>NKFITKDDEVIDYIYGKISPLFALQYIRKIDLKHVFEYDYHFEVNGTVVRHKNKGFGYMERFFELKESCDERSKLSKKQYERFNALFNFFEKNGVICMAKDAGTLNTSIEINSLAYHGKYDVMKKFIEEQSVSIEDDYKKAFFLACLGRWEESYDLYSNIILNSIDESNGCVYYLSQINRYRIYQSITQAVTQFNGLGLLTFGRHYKPFTDEFLARIEREMTNFNIDDLFNGMPFEFQKKYKILEFLSDNQFLYDDTVKLFELTNKVRSEMSEGSYSFGMSSDIVVLLRLYDNLRFLYENCLWSVSFHEFHQYIRNSMSLLIEKAEYERTRDIDELGFSFFGKKSGFFMEYYDFVNISRHFKIDDIKNLERSCSIDKIRFGEQEKIEEYLVGIAEEITKQFSANGMNVVFYTQFISEAKAALYFAKYVKLSEEGLGKIVKALLFYFPERDLDIGKRYVWLERLTKCNELPKSIISIIDDFLVLQAEKHIDQNYSEVSSNGLYSRDYGALIKHFEKNFISKRLSEITLCLTQDKQKQIDFLF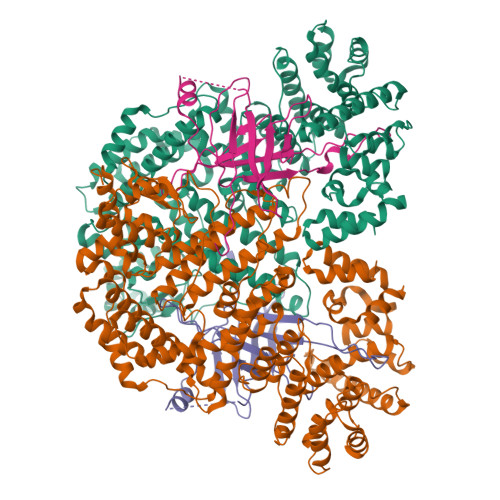KLLPLLSTNAKSHLLSFKSVENINDLMNGIRIGLIDEFTPEHEELIIEYLETRKVNYIVEKEKGIQTFSSNDYMSTFGIWYFLEEINNSKMEEFIGMDDQYDFFVDPENFDYKKFIPSWLKNYNDKLLGKIAGNKHMKHHVIEVLKERVKNSNDKRYLEILMNYFI[2x];>MKTVIQDTADVYFKRKSDGKLVFTAEAQTASFSQAISEEKLRGGIGNKPLYILKSEKEINLTVKNAFFDLEWLAMTQGETIQEETKVKVFDREHGLIVDDTNKVTLKGKPVSDVTFYNKKGLTYKIAVSTDGTYTIPTAFAAAKDKLTAVYQIEKVGRRLAIKASKFSERYEVEYRTIAYNPDTEEVYSDIYIQFPNVSPSGEFEMSLENGNALAPEIKFEALADTDTDEMAVVIEASRDENTAAPVEDTTGSTQSSDLGGTTE[2x]Zymogen granule membrane protein 16 (ZG16) is produced in organs that secrete large quantities of enzymes and other proteins into the digestive tract. ZG16 binds microbial pathogens, and lower ZG16 expression levels correlate with colorectal cancer, but the physiological function of the protein is poorly understood. One prominent attribute of ZG16 is its ability to bind glycans, but other aspects of the protein may also contribute to activity. An intriguing feature of ZG16 is a CXXC motif at the carboxy terminus.

Here, we describe crystal structures and biochemical studies showing that the CXXC motif is on a flexible tail, where it contributes little to structure or stability but is available to engage in redox reactions. ZG16 crystal structures also draw attention to a nonproline cis peptide bond that can isomerize within the protein and to the mobility of glycine‐rich loops in the glycan‐binding site. An understanding of the properties of the ZG16 CXXC motif and the discovery of internal conformational switches extend existing knowledge relating to the glycan‐binding activity of the protein.

> GARSSSYSGEYGSGGGKRFSHSGNQLDGPITALRVRVNTYYIVGLQVRYGKVWSDYVGGRNGDLEEIFLHPGESVIQVSGKYKWYLKKLVFVTDKGRYLSFGKDSGTSFNAVPLHPNTVLRFISGRSGSLIDAIGLHWDVYPSSCSRC N-[4-(aminomethyl)benzyl]-4-oxo-3,4-dihydrothieno[2,3-d]pyrimidine-5-carboxamide | C15 H14 N4 O2 S | 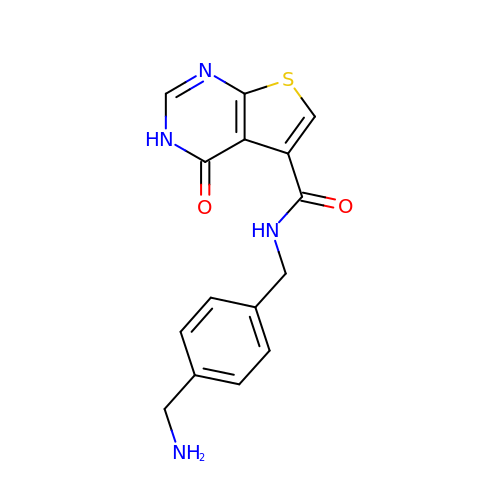ZOJIHHOGTNVURO-UHFFFAOYSA-N(7S)-8-(cyclopropylmethyl)-2-[(3,5-difluoro-4-hydroxyphenyl)amino]-7-methyl-5-(prop-2-yn-1-yl)-7,8-dihydropteridin-6(5H)-one | 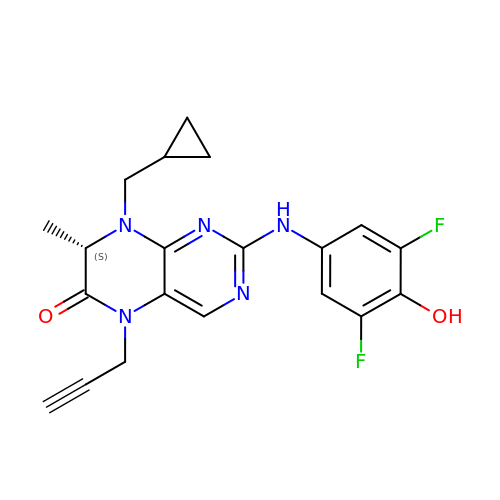C20 H19 F2 N5 O2 | VCABIQKTZQAYKL-NSHDSACASA-N>GCPRILIRCKQDSDCLAGCVCGPNGFCG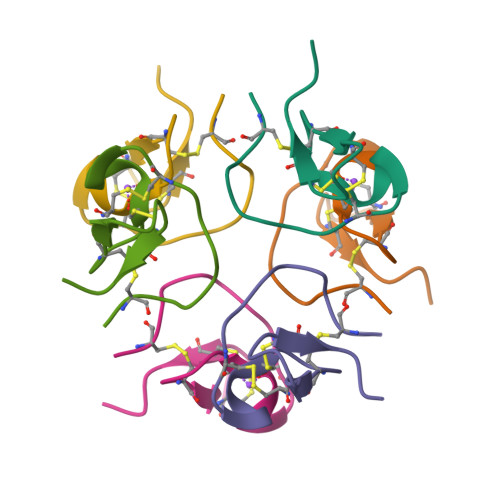SPA[8x]>GPHMGGSMQKVSLRVTPRLVLEVNRHNAICVATNVPEFYNARGDLNIRDLRAHVKARMISSQFCGYVLVSLLDSEDQVDHLNIFPHVFSERMILYKPNNVNLMEMCALLSMIENAKSPSIGLCREVLGRLTLLHSKCNNLDSLFLYNGARTLLSTLVKYHDLEEGAATPGPWNEGLSLFKLHKELKRAPSEARDLMQSLFLTSGKMGCLARSPKDYCADLNKEEDANSGFTFNLFYQDSLLTKHFQCQTVLQTLRRKCLGSDTVSKIIP[6x];>[6x]GPLGSECPDRWRAEIDLGLPPGVQVGDLLRNEQTMGSLRQVYLLAVQANSITDHLKRFDAVRVPE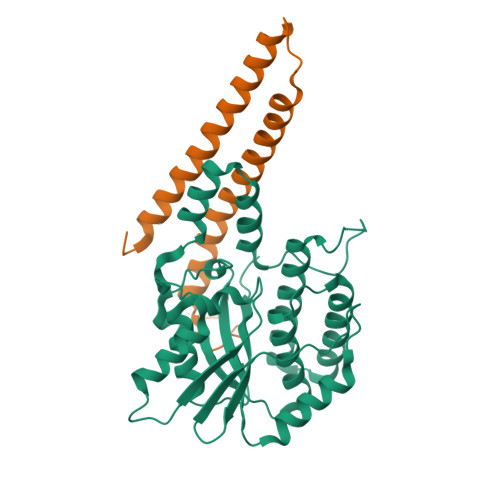SCRGVVEAQVAKLEAVRSVIWNTMISLAVSGIEMDENGLKALLDKQAGDSLALMEMEKVATALKMD>MQQLNPSEISALIKQRIGDLDTSATAKNEGTIVMVSDGIVRIHGLADAMYGEMIEFDGGLFGMALNLEQDSVGAVVLGNYLSLQEGQKARCTGRVLEVPVGPELLGRVVDALGNPIDGKGPIDAKLTDAVEKVAPGVIWRQSVDQPVQTGYKSVDTMIPVGRGQRELIIGDRQTGKTAMAIDAIIAQKNSGIKCVYVAIGQKQSTIANVVRKLEETGAMAYTTVVAAAAADPAAMQYLAPYSGCTMGEYFRDRGEDALIIYDDLSKQAVAYRQISLLLRRPPGREAYPGDVFYLHSRLLERASRVSAEYVEKFTNGAVTGKTGSLTALPIIETQAGDVSAFVPTNVISITDGQIFLETSLFNAGIRPAVNAGISVSRVGGSAQTKIIKKLSGGIRTALAQYRELAAFAQFASDLDEATRKQLEHGQRVTELMKQKQYAPYSIADQAVSVYASNEGYMADVEVKKIVDFDAALIAYFRSEYAPLMKQIDETGDYNKDIEAAIKAGIESFKATQTY[3x];>[3x]MSSGRIIQIIGAVIDVEFERTSVPKIYDALQVDGTETTLEVQQQLGDGVVRTIAMGSTEGLKRGLTVTSTNAPISVPVGTATLGRIMDVLGRPIDEAGPVATEERLPIHRQAPSYAEQAASTDLLETGIKVIDLLCPFAKGGKVGLFGGAGVGKTVNMMELINNIAKAHSGLSVFAGVGERTREGNDFYHEMKDSNVLDKVAMVYGQMNEPPGNRLRVALTGLTMAEYFRDEKDENGKGRDVLLFVDNIYRYTLAGTEVSALLGRMPSAVGYQPTLAEEMGVLQERITSTKSGSITSIQAVYVPADDLTDPSPATTFAHLDATVVLSRDIASSGIYPAIDPLDSTSRQLDPLVVGQEHYEIARAVQNVLQRYKELKDIIAILGMDELAEEDKLVVYRARKIQRFFSQPFHVAEVFTGAPGKLVPLKETIRGFKGLLAGEYDHIPEQAFYMVGGIDEVIAKAEKL;>MELTLGLVAIASAILIAFGALGTAIGFGLLGGRFLEAVARQPELAPQLQTRMFLIAGLLDAVPMIGVGIGLFFIFANPFVG[10x];> MAAEEHALTSTEYIKHHLTNMTYGKMPDGTWKLAETAEEAHSMGFTAIHLDSMGWSIGLGVIFCLLFWIVARAANAGVPTKFQSAIEMIIEFVDSSVRDTFHGKSRLIAPLALTIFVWIFLMNLMDLIPVDWIPQVAAFVGANVFGMDPHHVYFKIVPSTDPNITLGMSLSVFVLILFYSIREKGVGGFVGELALNPFNPSNPVAKALLIPVNLILELVTFLARPISLALRLFGNMYAGELIFILIALLPFWIQWALSVPWAIFHILVITLQAFIFMMLTIVYLSMASEKH;>[2x]MNINLTLIGQAIAFAFFVAFCMKFVWPPLINAISERQRKIADGLNAAEKAKADLADAQAQVKQELDAAKAQAAQLIEQANRRAAQLIEEARTQAAAEGERIRQQAKEAVDQEINSAREELRQQVAALAVTGAEKILNQQVDAEAHNAMLSQLAAKL;> MAELLTLARPYAKAAFAYASEQGATDNWSNALQVLSAAVQDEAFSAYLNRPELTPAEQVKLFAKVLGEDQSQAVSNFLTLLADNDRLVLLPEIAAEYEQLKSQNNNNVDVVIESAFPLTAEQEQLLKSALEKRFNSTVTVSVEVKPELIAGVVIRAGDQVIDDSALNKLEKMRTRLLA;> MATMQCDVVSVKESIYSGAVTMLIAKGAGGELGILPGHAPLVTLLQPGPIRVLLENGTEEIVYVSGGVLEVQPHVVTVLADTAIRADNLDEAAILEARKNAEQLLANQKSDLDSAAALAALAETAAQLETIRKIKNRAQ;> MANLKEIRAKVASIKSTQKITRAMQMVAASKMRRAQERMAQGRPYADNMRRVIAHLVQANPEYKHRYMVDRPVKRVGYIIVSSDRGLAGGLNINLFKKVVQHVKAQQEQSIEVQFALIGQKAVSFFKNYGGKVLGATTQIGDAPSLEQLTGSVQVMLDAFDKGELDRIYLVSNGFVNAMTQKPKVEQLVPLAPAEEGDDLNRTYGWDYIYEPEAEELLNGLLVRYIESMVYQGVIENVACEQSARMVAMKAATDNAGQLIKDLQLIYNKLRQAAITQEISEIVGGAAAV

F1Fo-ATP synthases are large, membrane-embedded macromolecular complexes that harness energy from the proton-motive force (pmf) and use it to synthesize ATP via a unique rotary mechanism. We solved the electron cryo-microscopy structure of the F1Fo–adenosine 5′-triphosphate (ATP) synthase from A. baumannii in three distinct conformational states. The A. baumannii ATP synthase has a subunit stoichiometry of α3β3γδεab2c10; its overall architecture resembles that of other bacterial and chloroplast ATP synthases. The rotating c-ring transfers torque to a central shaft comprising the ε- and γ-subunits, which protrude into the α3β3 hexamer, inducing conformational changes in the F1 nucleotide binding pockets, thus converting the rotary force into ATP synthesis.

State 1 was then used as a reference to build structures of the remaining two states. The central stalk is rotated by almost exactly 120o between each of the three conformational states suggesting common stable low-energy intermediate states in bacterial ATP synthases. Structural alignments of the γ-subunit between states revealed that the three states differ by almost exactly 120°.>[6x]GAMAPLQPGDSFPANVVFSYIPPTGSLDLTVSGRPIEYNASEALAKGTSVLVAVPGAFTPTCQEKHVTGFIAKLDQLRQAGVDRVLFIASNDAFVMSAWGKANGIKDESILFLSDSDTAFSSSIGWANAGRTGRYAIVVKDGKVVYAAVDTVRGSTEKSGVDAVLTVLGNQGKL;>MASSKAKLEEIPITVDFSGGLEMLFDNQRRHSISLPAKDTEGKPVTIAFLIDYISKKLMKDPRTDLFVLD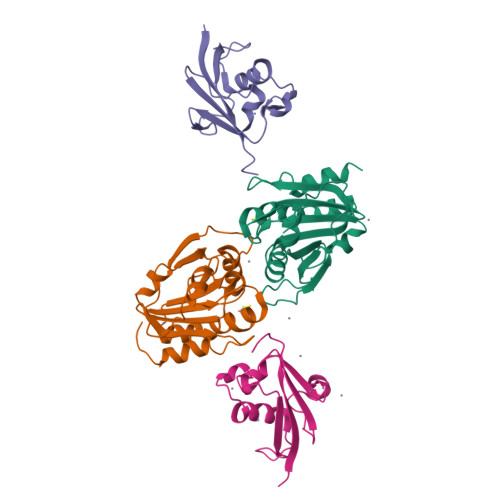NHIRPGILVLINDADWELEGEEAYEIQPNDNILFVSTLHGG[6x]>MAHHHHHHSSGLEVLFQGPNNTIINSLIGGDDSIKRSNVFAVDSQIPTLYMPQYISLSGVMTNDGPDNQAIASFEIRDQYITALNHLVLSLELPEVKGMGRFGYVPYVGYKCINHVSISSCNGVIWEIEGEELYNNCINNTIALKHSGYSSELNDISIGLTPNDTIKEPSTVYVYIKTPFDVEDTFSSLKLSDSKITVTVTFNPVSDIVIRDSSFDFETFNKEFVYVPELSFIGYMVKNVQIKPSFIEKPRRVIGQINQPTATVTEVHAATSLSVYTKPYYGNTDNKFISYPGYSQDEKDYIDAYVSRLLDDLVIVSDGPPTGYPESAEIVEVPEDGIVSIQDADVYVKIDNVP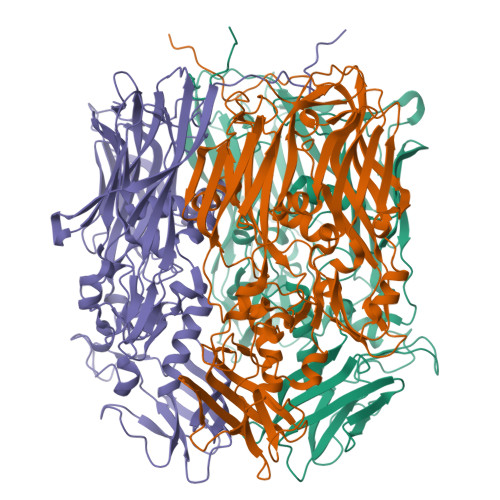DNMSVYLHTNLLMFGTRKNSFIYNISKKFSAITGTYSDATKRTIFAHISHSINIIDTSIPVSLWTSQRNVYNGDNRSAESKAKDLFINDPFIKGIDFKNKTDIISRLEVRFGNDVLYSENGPISRIYNELLTKSNNGTRTLTFNFTPKIFFRPTTITANVSRGKDKLSVRVVYSTMDVNHPIYYVQKQLVVVCNDLYKVSYDQGVSITKIMGDNN[3x]Before the glycosidases can act, the terminal glucosamine of HS must be acetylated by the integral lysosomal membrane enzyme heparan-α-glucosaminide N-acetyltransferase (HGSNAT). HGSNAT catalyzes a unique transmembrane acetylation reaction where the acetyl group of cytosolic acetyl-CoA is transported across the lysosomal membrane and attached to HS in one reaction. We find that a central pore within each monomer traverses the membrane and controls access of cytosolic acetyl-CoA to the active site at its luminal mouth where glucosamine binds. A histidine-aspartic acid catalytic dyad catalyzes the transfer reaction via a ternary complex mechanism.

To address these questions, we determined structures of both the substrates and products complexes. Acetyl-CoA binds in a linear fashion that traverses the entire TMD, while MU-βGlcN binds at the luminal mouth of the acetyl-CoA binding site with the amine group facing the acetyl group on acetyl-CoA. The CoA moiety interacts with HGSNAT through an extensive network of polar and hydrophobic interactions: a large number of polar interactions at the cytosolic mouth stabilize the 3’-phosphoadenosine, while R345 and R275 form hydrogen/ionic bonds with the diphosphate; the pantothenate group is accommodated through hydrophobic interactions, while the cysteamine forms a hydrogen bond with M282. The carbonyl of the acetyl group is stabilized by N286, whose mutation is identified in MPS patients. The GlcN moiety’s interaction with the luminal cavity formed by the ECLs is mediated mostly by polar interactions, including with the proposed catalytic residue H29711,17. R372 and E499, whose mutations lead to low activity and mis-localization of HGSNAT in MPS patients, bind to the 6’-OH and 3’-OH of GlcN respectively. We identified a catalytic dyad of H297-D307 in the structures, which lowers the pKa of H297 to ~ 4, as calculated by PROPKA21. Meanwhile, H297 is positioned within a distance that would allow it to deprotonate the amine of GlcN. In addition, N286 is positioned 2.7 Å away from the carbonyl oxygen of the acetyl group, which stabilizes the negative charge in the intermediate state. We observed slightly different configurations of the active site between the two monomers where one monomer appears to have bonding distances better suited for catalysis than the other, suggesting that the two monomers may be in active state asynchronously.

>[2x]MTGARASAAEQRRAGRSGQARAAERAAGMSGAGRALAALLLAASVLSAALLAPGGSSGRDAQAAPPRDLDKKRHAELKMDQALLLIHNELLWTNLTVYWKSECCYHCLFQVLVNVPQSPKAGKPSAAAASVSTQHGSILQLNDTLEEKEVCRLEYRFGEFGNYSLLVKNIHNGVSEIACDLAVNEDPVDSNLPVSIAFLIGLAVIIVISFLRLLLSLDDFNNWISKAISSRETDRLINSELGSPSRTDPLDGDVQPATWRLSALPPRLRSVDTFRGIALILMVFVNYGGGKYWYFKHASWNGLTVADLVFPWFVFIMGSSIFLSMTSILQRGCSKFRLLGKIAWRSFLLICIGIIIVNPNYCLGPLSWDKVRIPGVLQRLGVTYFVVAVLELLFAKPVPEHCASERSCLSLRDITSSWPQWLLILVLEGLWLGLTFLLPVPGCPTGYLGPGGIGDFGKYPNCTGGAAGYIDRLLLGDDHLYQHPSSAVLYHTEVAYDPEGILGTINSIVMAFLGVQAGKILLYYKARTKDILIRFTAWCCILGLISVALTKVSENEGFIPVNKNLWSLSYVTTLSSFAFFILLVLYPVVDVKGLWTGTPFFYPGMNSILVYVGHEVFENYFPFQWKLKDNQSHKEHLTQNIVATALWVLIAYILYRKKIFWKI>MAKILEGPAMKLFNKWGIPVPNYVVIMDPDRLAQLGEANKWLRESKLVVKAHEAIGGRFKLGLVKIGLNLEQAIEAAKEMLGAKVGTAEIGQVIIAEMLEHDAEFYVSIIGNKDGAELLISKHGGVDIEDNWDSVRRIQIELDENPTIEQLTELAKDAGFEGEIAERVGKICSRLILCFDNEDAQSIEINPLVIRKSDMRFAALDAVMNVDYDARFRHADWDFKPVSEIGRPFTEAEQQIMEIDSRIKGSVKFVEVPGGEIALLTAGGGASVFYADAVVARGGTIANYAEYSGDPADWAVEALTETICRLPNIKHIIVGGAIANFTDVKATFSGIINGFRESKSKGYLEGVKIWVRRGGPNEAQGLAAIKQLQEEGFDIHVYDRSMPMTDIVDLAMKS[4x];>[4x]MSILANKDTRAVIIGGVAGVNAAKRMAQFDFLVNRPLTVQAFVYPPEAGQQKEIFRGGELKNVTVYDSLAPALEEHPDINTALIYLGASRAAQAAKEALESPNIQLVSMITEGVPEKDAKRLKKLAQKLGKMLNGPSSIGIMSAGECRLGVIGGEFKNLKLCNLYRQGSFGVLTKSGGLSNEAMWLCAQNGDGITSAVAIGGDAYPGTDFVTYLEMFEKDPATKAVVMIGEVGGNLEEEAAEWLAAEPRRIKLIAAIGGTCQEVLPQGMKFGHAGAKEGKKGAGSARSKMNALRDAGAYVPDTFGGLSK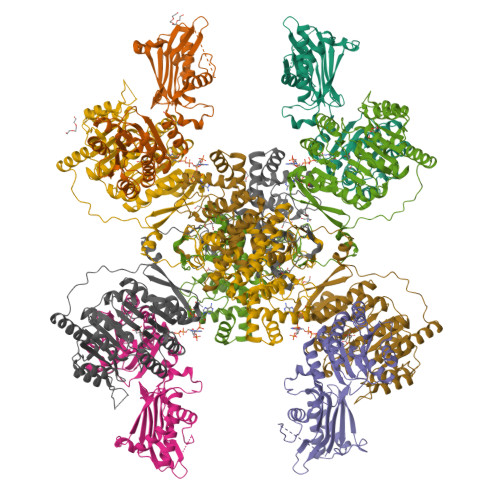EIKKVYEELIAAGEISTEIDEAVLPELPPRVQEVMKQGEVIVEPLIRTTISDDRGEEPRYAGYAASELCSKGYGIEDVIGLLWNKKLPTREESEIIKRIVMISADHGPAVSGAFGSILAACAGIDMPQAVSAGMTMIGPRFGGAVTNAGKYFKMAVEDYPNDIPGFLSWMKKNVGPVPGIGHRVKSVKNPDQRVKYLVSYIKNETSLHTPCLDYALEVEKVTTAKKGNLILNVDGTIGCILMDLDFPVHSLNGFFVLARTIGMIGHWIDQNNQNSRLIRLYDYLINYAVKPEQEVPEKKGGSHHHHHH>MTLEQAIERAGTKHGNKGWEAALSAIEMANLFKSLRGTGGSGSSMEIYEGKLTAEGLRFGIVASRFNHALVDRLVEGAIDCIVRHGGREEDITLVRVPGSWEIPVAAGELARKEDIDAVIAIGVLIRGATPHFDYIASEVSKGLANLSLELRKPITFGVITA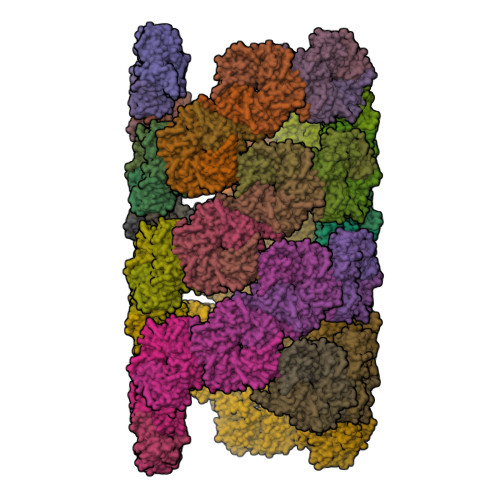D[150x]>[24x]SNAMGLDVRNNGNDNVEIRAAETRTAQRADEALETAADFAGQPKVTHTMRTINRTLSRRISRNTGSEQVLNLRRLMEKYLEDTRFKDDFIFVAVDPNQYSVPYPTLVVMSGAKVGDHNHFFGYVLPLVAGLAPLPRREEQGPHGNILVPRTWVDNLNGTFINEVMAAMYAAIGGKSNGTARIAGLAVVTNEITAESAHLAT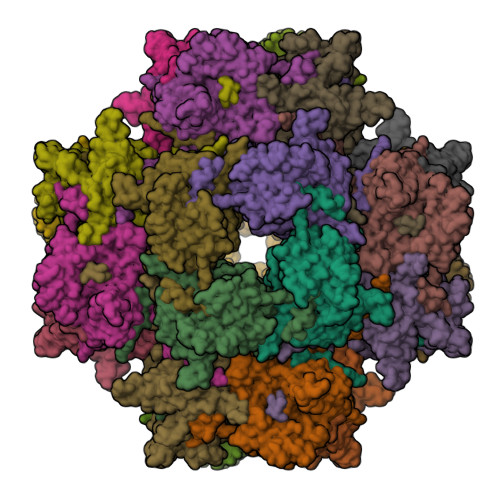TLLSAADNAIQTAIEIRLGDKLGLPQFNLGMMASDQPISSVQYNTSGMQDSDIVGNPVRSDITVTISNRIRQAMSDYDSQQRLVATTGYIDLTYSPQNPTFNQGPVLVNGYPVPPTVQYQPRYVMTSAYPLELDAFTPNTFVLGLIGTIATLNSGMAWAQSLISNAARGIGPHNPGALAMVLDPEVTAPLDLSTQTNEQIYKFLQQVLYPSLLISIDVPEEGEYSWLLRMIPAAEKIYTGKVEGEVREISEGYKALYRAFDDVTLGCFSKKYQYGLPLVYATGNRIPLGHYNHQDGHRHDIRDMDDLYMMNITNPDTVEAWEDSFDRTDMTMSQRVVARHEIIDRVLSGSWEQTGWAMRYDFDPLALQALIEAAADAGFTIRPENIQHLAGTAVRGNMAARARGLGNISGNIYARSDRPNVGVNNMGGAFNLF>GSRKIIHVDMDCFFAAVEMRDNPALRDIPIAIGGSRERRGVISTANYPARKFGVRSAMPTGMALKLCPHLTLLPGRFDAYKEASNHIREIFSRYTSRIEPLSLDEAYLDVTDSVHCHGSATLIAQEIRQTIFNELQLTASAGVAPVKFLAKIASDMNKPNGQFVITPAEVPAFLQTLPLAKIPGVGKVSAAKLEAMGLRTCGDVQKCDLVMLLKRFGKFGRILWERSQGIDERDVNSERLRKSVGVERTMAEDIHHWSECEAIIERLYPELERRLAKVKPDLLIARQGVKLKFDDFQQTTQEHVWP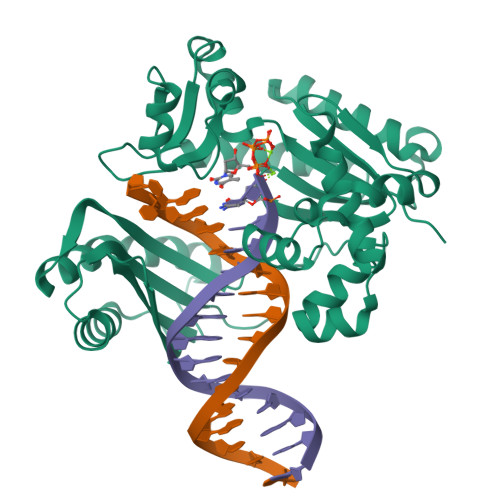RLNKADLIATARKTWDERRGGRGVRLVGLHVTLLDPQMERQLVLGL[2x]>[2x]MKTVTVKNLIIGEGMPKIIVSLMGRDINSVKAEALAYREATFDILEWRVDHFMDIASTQSVLTAARVIRDAMPDIPLLFTFRSAKEGGEQTITTQHYLTLNRAAIDSGLVDMIDLELFTGDADVKATVDYAHAHNVYVVMSNHDFHQTPSAEEMVLRLRKMQALGADIPKIAVMPQSKHDVLTLLTATLEMQQHYADRPVITMSMAKEGVISRLAGEVFGSAATFGAVKQASAPGQIAVNDLRSVLMILHNA

Several studies have identified the enzyme type I dehydroquinase (DHQ1, 3-dehydroquinate dehydratase, EC 4.2.1.10) as a promising target for anti-virulence drug development. DHQ1 catalyzes the reversible dehydratation of 3-dehydroquinic acid (1) to 3-dehydroshikimic acid (2), which is the third step in the shikimic acid pathway. It follows a covalent catalysis mechanism with the formation of transient Schiff base species´ between the ketone moiety of the substrate and the ɛ-amino group of a catalytic lysine residue (K160/K170 in Sa-DHQ1 and St-DHQ1, respectively), which are finally hydrolyzed to regenerate the enzyme. An essential histidine residue (H133/H143 in Sa-DHQ1 and St-DHQ1, respectively), is also involved in the formation/hydrolysis of the Schiff base intermediates.

Herein we report the synthesis of compounds 6–7 in which enhancement of the electrophilicity of an endocyclic carbon atom in the ligand towards covalent modification is attempted by direct introduction of the amino functionality into the quinate scaffold. These compounds are substrate analogs in which the carbonyl group at C3 has been replaced by a hydroxyamino and an amino group with R configuration (compounds 6 and 7, respectively). Compound 6 was found to be a time-dependent irreversible inhibitor of the two enzymes with K I values of 90 ± 8 and 130 ± 12 µM and k inact values of 8 ± 1 and 13 ± 1 ms−1 against Sa-DHQ1 and St-DHQ1, respectively. The two adducts Sa-DHQ1/6 and St-DHQ1/6 crystallized as dimers with two molecules in the asymmetric unit (namely chains A and B) and were solved at a resolution of 1.65 and 1.90 Å, respectively. Unbiased, calculated electron-density maps showed clear electron density for the ligand covalently bonded to the catalytic lysine residue (K160/K170 in Sa-DHQ1 and St-DHQ1, respectively) via an amine, which is visible in the two chains. Surprisingly, no electron density for the tertiary hydroxyl group in position C1 was identified in the two enzyme adducts. Dehydration involving the C1–C2 bond took place to give a shikimate-like core, perhaps after covalent linkage at the C3 position in 6 via a similar mechanism to that observed for the natural substrate. Thus, compound 6 provides non-labile enzyme adducts by avoiding the intrinsic Schiff base hydrolysis performed by the enzyme. For the St-DHQ1/6 enzyme adduct, a long hydrogen bond between the C5 hydroxyl group and the side chain of residue S21, which is located on the flexible substrate-covering loop, is also identified. As a result, this loop folds more above the modified ligand. The MALDI spectra of St-DHQ1 enzyme incubated with 6 in ∼1:120 enzyme/ligand ratio for 24 h and at 25°C showed a peak for a covalently modified enzyme corresponding to an additional mass of 158 (theoretical value of the increased mass = 156).>[12x]AFFTTVIIPAIVGGIATGTAVGTVSGLLGWGLKQAEEANKTPDKPDKVWRIQAGKGFNEFPNKEYDLYKSLLSSKIDGGWDWGNAATHYWIKGGQWNKLEVDMKDAVGTYKLSGLRNFTGGDLDVNMQKATLRLGQFNGNSFTSYKDSADRTTRVDFNAKNILIDNFLEINNRVGSGAGRKASSTVLTLQASEGITSSKNAEISLYDGATLNLASNSVKLNGNVWMGRLQYVGAYLAPSYSTINTSKVTGEVNFNHLTVGDHNAAQAGIIASNKTHIGTLDLWQSAGLNIIAPPEGGYKDKPNNTPSQSGAKNDKQESSQNNSNTQVINPPN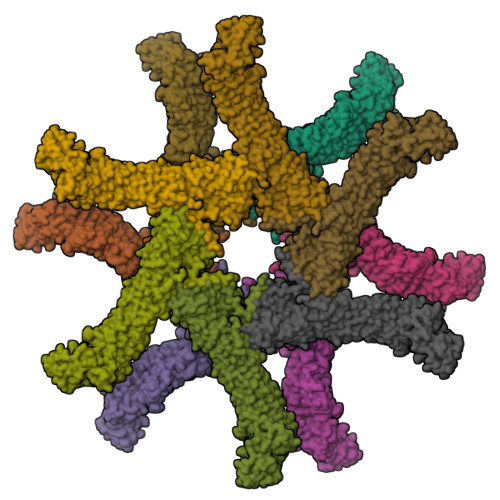STQKTEVQPTQVIDGPFAGGKDTVVNIDRINTKADGTIKVGGFKASLTTNAAHLNIGKGGVNLSNQASGRTLLVENLTGNITVDGPLRVNNQVGGYALAGSSANFEFKAGVDTKNGTATFNNDISLGRFVNLKVDAHTANFKGIDTGNGGFNTLDFSGVTNKVNINKLITASTNVAVKNFNINELIVKTNGVSVGEYTHFSEDIGSQSRINTVRLETGTRSIFSGGVKFKSGEKLVIDEFYYSPWNYFDARNIKNVEITRKFASSTPENPWGTSKLMFNNLTLGQNAVMDYSQFSNLTIQGDFINNQGTINYLVRGGKVATLNVGNAAAMMFNNDIDSATGFYKPLIKINSAQDLIKNTEHVLLKAKIIGYGNVSTGTNGISNVNLEEQFKERLALYNNNNRMDTCVVRNTDDIKACGMAIGNQSMVNNPDNYKYLIGKAWKNIGISKTANGSKISVYYLGNSTPTENGGNTTNLPTNTTNNARFASYA> MKIYVDGREVIINDNERNLLEALKNVGIEIPNLCYLSEASIYGACRMCLVEINGQITTSCTLKPYEGMKVKTNTPEIYEMRRNILELILATHNRDCTTCDRNGSCKLQKYAEDFGIRKIRFEALKKEHVRDESAPVVRDTSKCILCGDCVRVCEEIQGVGVIEFAKRGFESVVTTAFDTPLIETECVLCGQCVAYCPTGALSIRNDIDKLIEALESDKIVIGMIAPAVRAAIQEEFGIDEDVAMAEKLVSFLKTIGFDKVFDVSFGADLVAYEEAHEFYERLKKGERLPQFTSCCPAWVKHAEHTYPQYLQNLSSVKSPQQALGTVIKKIYARKLGVPEEKIFLVSFMPCTAKKFEAEREEHEGIVDIVLTTREL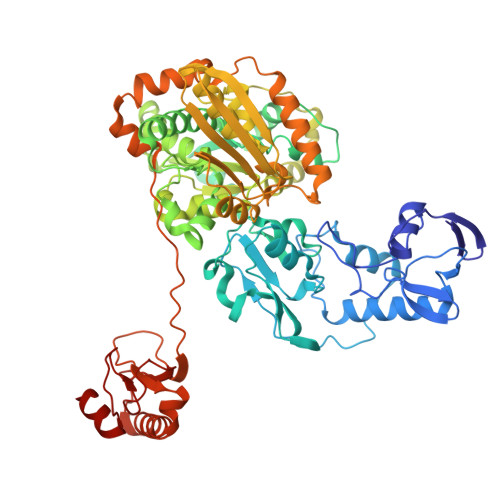AQLIKMSRIDINRVEPQPFDRPYGVSSQAGLGFGKAGGVFSCVLSVLNEEIGIEKVDVKSPEDGIRVAEVTLKDGTSFKGAVIYGLGKVKKFLEERKDVEIIEVMACNYGCVGGGGQPYPNDSRIREHRAKVLRDTMGIKSLLTPVENLFLMKLYEEDLKDEHTRHEILHTTYRPRRRYPEKDVEILPVPNGEKRTVKVCLGTSCYTKGSYEILKKLVDYVKENDMEGKIEVLGTFCVENCGASPNVIVDDKIIGGATFEKVLEELSKNG> TENLDNVALSSSPIHSGFLVSFMVDARGGAMRGCRHNGLRIIIPPRKCTAPTRVTCRLVKRHRLATMPPMVEGEGLASRLIEVGPSGAQFLGPVIVE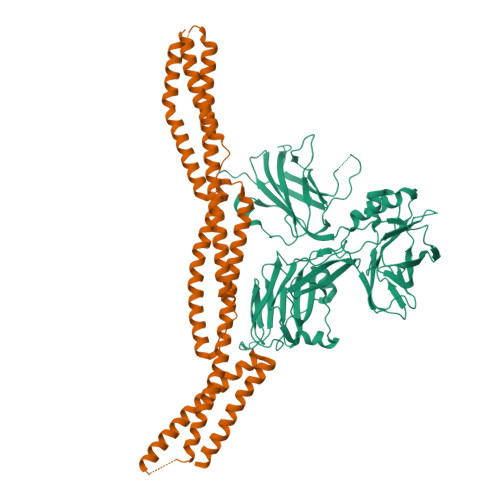IPHFAALRGKERELVVLRSENGDSWKEHFCDYTEDELNEILNGMDEVLDSPEDLEKKRICRIITRDFPQYFAVVSRIKQDSNLIGPEGGVLSSTVVPQVQAVFPEGALTKRIRVGLQAQPMHSELVKKILGNKATFSPIVTLEPRRRKFHKPITMTIPVPKASSDVMLNGFGGDAPTLRLLCSITGGTTPAQWEDITGTTPLTFVNECVSFTTNVSARFWLIDCRQIQESVTFASQVYREIICVPYMAKFVVFAKSHDPIEARLRCFCMTDDKVDKTLEQQENFAEVARSRDVEVLEGKPIYVDCFGNLVPLTKSGQHHIFSFFAFKENRLPLFVKVRDTTQEPCGRLSFMKEPKSTRGLVHQAICNLNITLPIYTKE;> AFQVEQYYFDVAEVEAWLGEQELLMMSEDKGKDEQSTLQLLKKHLQLEQGVENYEESIAQLSRQCRALLEMGHPDSEQISRRQSQVDRLYVALKELGEERRVSLEQQYWLYQLSRQVDELEHWIAEKEVVAGSPELGQDFEHVSVLQEKFSEFASETGTAGRERLAAVNQMVDELIECGHTAAATMAEWKDGLNEAWAELLELMGTRAQLLAASRELHKFFSDARELQGQIEEKRRRLPRLTAPPEPRPSASSMQRTLRAFEHDLQLLVSQVRQLQEGAAQLRTVYAGEHAEAIASREQEVLQGWKELLAACEDARLHVSST> MELAEKDKGRDFTLRNARMDDIDQIIKINRLTLPENYPYYFFVEHLKEYGLAFFVAIVDNSVVGYIMPRIEWGFSNIKQLPSLVRKGAVVSIAVLEEYRRKGIATTLLEASMKSMKNDYNAEEIYLAVRVSNYPAIALYEKLNFKKV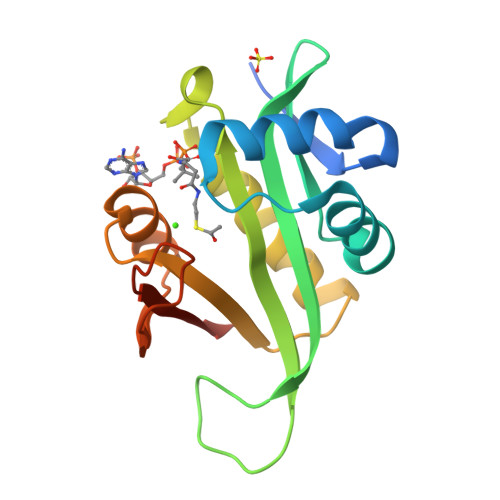KVLKGYYADGEDAYLMARPLHHHHHH>[2x]SNAMTKQYDYIVIGGGSGGIASANRAAMHGAKVILFEGKQVGGTCVNVGCVPKKV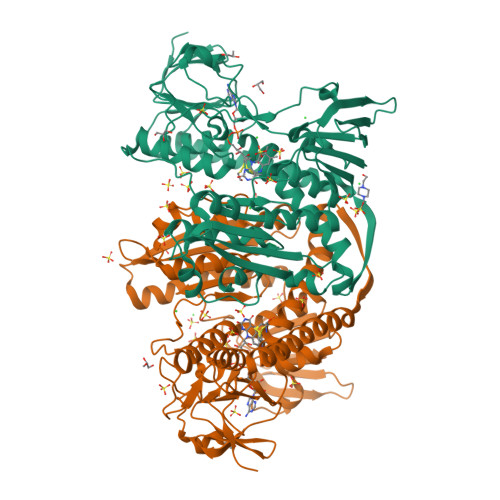MWYGAQVAETINNYAADYGFDVTTQAFHFDVLKQNRQAYIDRIHDSYERGFDSNGVERVYGYATFVDAHTVEVAGEHYTAPHILIATGGHALLPDIPGSEYGITSDGFFELDAIPKRTAVVGAGYIAVEISGILHALGSETHLFVRRDRPLRKFDKEIVGTLVDEMKKDGPHLHTFSVPKEVIKNTDNSLTLILENGEEYTVDTLIWAIGRAANTKGFNLEVTGVTLDSRGFIATDAFENTNVEGLYALGDVNGKLELTPVAVKAGRQLSERLFNHKPQAKMDYKDVATVIFSHPVIGSIGLSEEAALDQYGEENVTVYRSTFTSMYTAVTSHRQACKMKLVTVGEDEKIVGLHGIGYGVDEMIQGFAVAIKMGATKADFDNTVAIHPTGSEEFVTMR>[2x]MRVLGIETSCDETGIAIYDDEKGLLANQLYSQVKLHADYGGVVPELASRDHVRKTVPLIQAALKESGLTAKDIDAVAYTAGPGLVGALLVGATVGRSLAFAWDVPAIPVHHMEGHLLAPMLEDNPPEFPFVALLVSGGHTQLISVTGIGQYELLGESIDDAAGEAFDKTAKLLGLDYPGGPLLSKMAAQGTAGRFVFPRPMTDRPGLDFSFSGLKTFAANTIRDNGTDDQTRA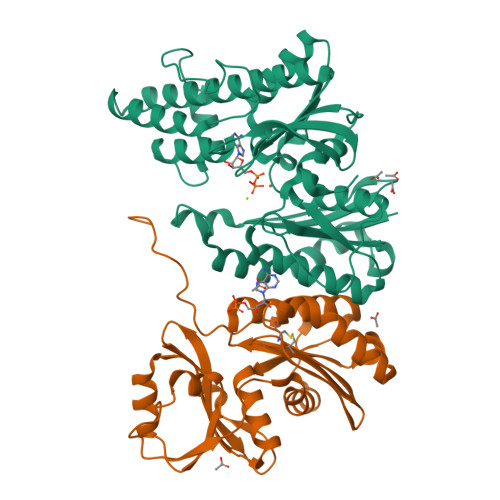DIARAFEDAVVDTLMIKCKRALDQTGFKRLVMAGGVSANRTLRAKLAEMMKKRRGEVFYARPEFCTDNGAMIAYAGMVRFKAGATADLGVSVRPRWPLAELPAAHHHHHH;>MRILAIDTATEACSVALWNDGTVNAHFELCPREHTQRILPMVQDILTTSGTSLTDINALAYGRGPGSFTGVRIGIGIAQGLALGAELPMIGVSTLMTMAQGAWRKNGATRVLAAIDARMGEVYWAEYQRDENGIWHGEETEAVLKPEIVHERMQQLSGEWVTVGTGWQAWPDLGKESGLVLRDGEVLLPAAEDMLPIACQMFAEGKTVAVEHAEPVYLRNNVAWKKLPGKEHHHHHH[2x]> GSLDGPYAPDSSNLPSNCWYLVNPSNDGVVFSVTDNSTFWMFTYLVLPNTAQTNVTVNVMNETVNISIDNSGSTYRFVDYIKTSSTQAYGSRNYLNTAHRLQAYRRDGDGNISNYWGADTQGDLRVGTYSNPVPNAVINLNADFYVIPDSQQETCTEYIRGGL

For rotaviruses (RVs), which are the major causative agents of life-threatening gastroenteritis in children under the age of 5 years and result in 453,000 deaths worldwide annually, recognition of specific cellular glycans for initial cell attachment is mediated by the distally located VP8* domain of the spike protein VP4. Although structurally conserved with a galectin-like fold, sequence-wise VP8* is the least conserved among RV structural proteins contributing to a phylogeny consisting of 37 [P] genotypes9. Our crystallographic analyses provide the structural basis to explain the unique glycan specificity exhibited by a neonate-specific bovine-human reassortant RV strain and its parental bovine strain, each belonging to the P genotype. We have shown that P VP8* exhibits a novel glycan-binding site that adapts to a differential recognition of precursor glycans, which are the core elements of HBGA and human/bovine milk glycans.

Sequence comparison of human and bovine P VP8*s shows 86% amino-acid identity. However, there are several significant amino acid changes from human to bovine P, including S180A, Y183Q, I158N and F192S. To investigate whether the sequence variations within the VP8*s of the same genotype lead to any structural changes, and how they account for differential glycan binding, we determined the crystal structure of VP8* from a P BRV strain B223 at 2.2 Å resolution. Comparison of the human and bovine P VP8* structures shows that despite the overall structural similarity (RMSD=0.66 Å), the J-K loop in the bovine VP8*, which has several sequence alterations undergoes significant structural change. In the bovine VP8*, this loop with a different set of inter-residue hydrogen bonds projects in an opposite direction compared with that of the human VP8*. The backbone conformational angles in this loop from residues G179 to G184 are also significantly altered. Comparative analysis clearly shows that the amino acid changes S180A, Y183Q, I158N along with the altered conformation of the J-K loop in the bovine VP8* result in the loss of the binding pocket for type I Galβ1,3-GlcNAc motif. The residue Y183 in the human VP8* that is involved in a stabilizing hydrophobic stacking interaction with the type I glycan is replaced by Q183 in the bovine VP8*, which in the structure is shifted 5.3 Å away because of the conformational change in the J-K loop. S180, which interacts with β1,3-linked GlcNAc of LNT through stabilizing hydrophobic and hydrogen-bonding interactions, is replaced by A180, which based on the superposition of the structures clashes with this moiety. In addition, I158 that is involved in a hydrophobic interaction with GlcNAc in the human VP8* is replaced by a hydrophilic residue N158.> GSRSGVAVADESLTAFNDLKLGKKYKFILFGLNDAKTEI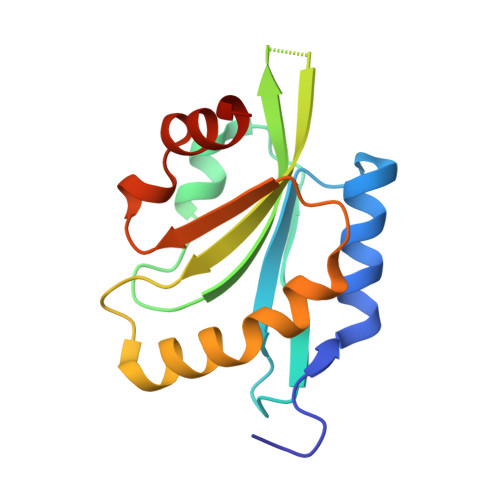VVKETSTDPSYDAFLEKLPENDCLYAIYDFEYEINGNEGKRSDIVFFTWSPDTAPVRSKMVYASSKDALRRALNGVSTDVQGTDFSEVSYDSVLERVSRGAGSH>[2x]FQGAMDPEFSMKIGIIGAMEEEVTLLRDKIENRQTISLGGCEIYTGQLNGTEVALLKSGIGKVAAALGATLLLEHCKPDVIINTGSAGGLAPTLK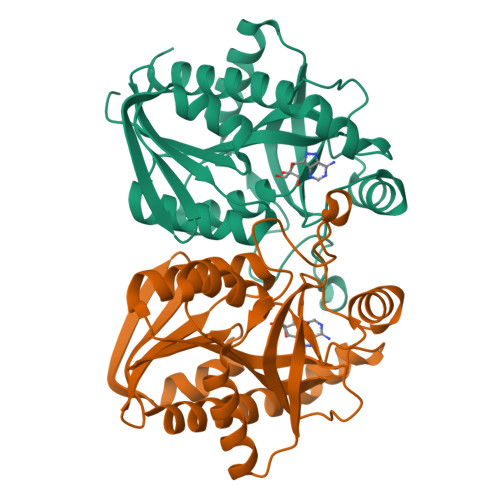VGDIVVSDEARYHDADVTAFGYEYGQLPGCPAGFKADDKLIAAAEACIAELNLNAVRGLIVSGDAFINGSVGLAKIRHNFPQAIAVEMEATAIAHVCHNFNVPFVVVRAISDVADQQSHLSFDEFLAVAAKQSSLMVESLVQKLAHG> GSMYVIRDEWGNQIWICPGCNKPDDGSPMIGCDDCDDWYHWP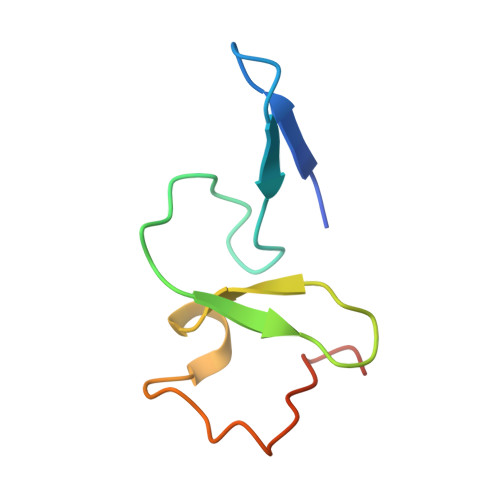CVGIMTAPPEEMQWFCPKCANK> EEYVGLS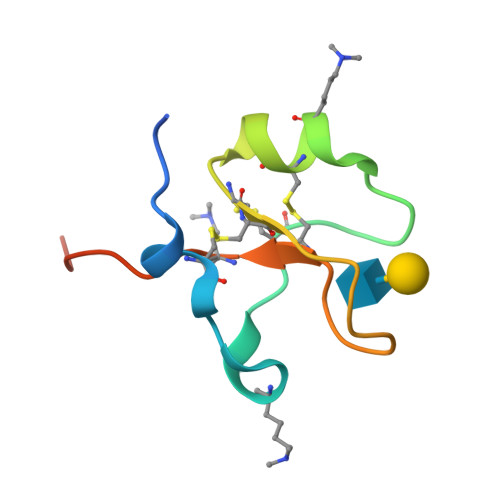ANQCAVPAKDRVDCGYPHVTPKECNNRGCCFDSRIPGVPWCFKPLQEAESTLEK> GMSGTANSRRKEVLRVPVIDLNRVSDEEQLLPVVRAILLQHDTFLLKNYANKAVLDALLAGLTTKDLPDTSQGFDANFTGTLPLEDDVWLEQYIFDTDPQLRFDRKCRNESLCSIYSRLFKLGLFFAQLCVKSVVSSAELQDCISTSHYATKLTRYFNDNGSTHDGADAGATVLPTGDDFQYLFERDYVTFLPTGVLTIFPCAKAIRYKPSTMATTDNSWVSIDEPDCLLFHTGTLLARWSQGMHTTSPLQIDPRANIVSLTIWPPLTTPISSKGEGTIANHLLEQQIKAFPKVAQQYYPRELSILRLQDAMKFVKELFTVCETVLSLNALSRSTGVPPELHVLLPQISSMMKRKIVQDDILKLLTIWSDAYVVELNSRGELTMNLPKRDNLTTLTNKSRTLAFVERAESWYQQVIASKDEIMTDVPAFKINKRRSSSN

The process of eukaryotic DNA replication begins during G1 phase with the loading of the minichromosome maintenance (MCM) heterohexamer comprising Mcm2–7 subunits into head-to-head double hexamers with double-stranded DNA passing through the length of a long central channel. This topological loading requires the Origin Recognition Complex (ORC), Cdc6 and Cdt1 proteins. In budding yeast, Cdt1 forms a stable complex with MCM before loading. We propose that Cdt1 stabilizes a conformation of the MCM ring in which the Mcm2–5 gate is held open to allow duplex DNA passage required for helicase loading. To understand Cdt1–MCM at an atomic level, we determined crystal structures of two non-overlapping fragments of S. cerevisiae Cdt1 spanning amino acid residues 1–438 and 495–604.

The structure of Cdt1(1–438) was refined using two independent crystal forms to resolutions of 2.7 and 2.1 Å. The fragment comprises a pair of well-defined domains corresponding to the N domain (residues 14–298) and the M domain (residues 299–430). The relative orientation between the domains is preserved in all four crystallographically independent copies of the protein chain observed in the crystal structures, indicating a rigid linkage between the domains. Perusal of the Dali structure comparison server revealed a striking similarity between the Cdt1 N domain and Fe(II)/α-ketoglutarate-dependent dioxygenase superfamily of enzymes, such as AlkB and other DNA/RNA dealkylators, and the Jumonji C histone demethylase21. However, the key His and Asp residues involved in chelation of the Fe(II) ion co-factor in the active sites of these enzymes are not conserved in the Cdt1 N domain. Moreover, an α-helical hairpin (α6/α7), which extends the dioxygenase fold, occludes the degenerate active site of the N domain. These observations indicate that the dioxygenase structural fold was repurposed for a non-catalytic function. By docking the crystal structure of NM Cdt1 into the Cdt1 density, an MCM interaction can be modelled, whereby the middle domain of Mcm2 is sandwiched between the A-domain and AAA+ domain of Mcm2 and extends to contact the A-domain of Mcm6, following the outer perimeter of the MCM N-terminal domain. Conversely, the N domain of Cdt1 projects away from the MCM ring and does not appear to be involved in any contact with the helicase motor. The N domain of the yeast protein plays an important role in MCM loading, but makes little or no contact with MCM in our structure.In human mitochondria, mitochondrial Hsp70 (mortalin) and the nucleotide exchange factor (GrpEL1) work synergistically to stabilize proteins, assemble protein complexes, and facilitate protein import. In bacteria, mitochondria, and chloroplasts, the GrpE-family of NEFs interacts with substrate-bound Hsp70 to facilitate ADP and protein substrate release. Herein, we present structures of full-length human mortalin in a nucleotide-free and substrate-bound state in complex with full-length GrpEL1. To stabilize the complex for structural analysis, we introduced a point mutation, R126W, into mortalin (mortalinR126W) that is associated with EVEN-PLUS syndrome and has been shown to reduce mortalin’s ATPase activity and conformational flexibility.

Further refinement yielded a 2.96 Å resolution cryoEM map describing a complex consisting of full-length mortalinR126W bound to a protein substrate and a full-length GrpEL1 homodimer. Firstly, we observe an expanded NBD devoid of nucleotide that is mediated by extensive contacts with one protomer of GrpEL1, termed GrpEL1-A. Secondly, we detail the significant bending of the GrpEL1 α-helical stalk domain that enables interactions between the GrpEL1 stalk and mortalinR126W NBD and SBD. Finally, this structure provides insights into the interactions between the SBDα helical lid of mortalin and the second GrpEL1 protomer, GrpEL1-B. Critically, the lack of EM density within the nucleotide-binding pocket but strong density within the substrate-binding pocket suggests that our structure represents a previously unobserved intermediate state and suggests a step-wise mechanism for the nucleotide and substrate release action of GrpEL1. At the first interface, subdomain IB of the NBD contacts the β-wing domain of GrpEL1-A via a salt bridge between R107 in mortalinR126W and the carbonyl group of P172 in GrpEL1-A. Here, the mortalinR126W IDL is proximal to the GrpEL1 α-helical dimer with residues V435 and L438 within the hydrophobic IDL interacting with L82 in GrpEL1-B. Compared to the predicted GrpEL1 structure, our mortalinR126W-GrpEL1 structure exhibits a ~ 13° bending of the GrpEL1 α-helical domain. We observed strong density for a peptide bound to the SBD substrate binding pocket, indicating that our purified complex is substrate-bound. With these factors in mind, combined with Hsp70’s propensity to bind hydrophobic peptides, we modeled the bound peptide as VLLLDVT, corresponding to residues 435–441 of mortalin’s IDL region, into our cryoEM density. Second, we observe an interaction interface between the SBDα helical domain and the β-wing domain of GrpEL1-B. Here, Y173 from GrpEL1-B inserts itself into the mortalinR126W SBDα, forming electrostatic and cation-pi stacking interactions with R578 and R574, respectively.

> MASEAIKGAVVGIDLGTTNSCVAVMEGKQAKVLENAEGARTTPSVVAFTADGERLVGMPAKRQAVTNPNNTFYATKRLIGWRYDDPEVQKDIKNVPFKIVRASNGDAWVEAHGKLYSPSQIGAFVLMKMKETAENYLGHTAKNAVITVPAYFNDSQRQATKDAGQISGLNVLRVINEPTAAALAYGLDKSEDKVIAVYDLGGGTFDISILEIQKGVFEVKSTNGDTFLGGEDFDQALLRHIVKEFKRETGVDLTKDNMALQRVREAAEKAKCELSSSVQTDINLPYLTMDSSGPKHLNMKLTRAQFEGIVTDLIRRTIAPCQKAMQDAEVSKSDIGEVILVGGMTRMPKVQQTVQDLFGRAPSKAVNPDEAVAIGAAIQGGVLAGDVTDVLLLDVTPLSLGIETLGGVFTKLINRNTTIPTKKSQVFSTAADGQTQVEIKVCQGEREMAGDNKLLGQFTLIGIPPAPRGVPQIEVTFDIDANGIVHVSAKDKGTGREQQIVIQSSGGLSKDDIENMVKNAEKYAEEDRRKKERVEAVNMAEGIIHDTETKMEEFKDQLPADECNKLKEEISKMRELLARKDSETGENIRQAASS;>[2x]TLLEEKVKLEEQLKETVEKYKRALADTENLRQRSQKLVEEAKLYGIQAFCKDLLEVADVLEKATQCVPKEEIKDDNPHLKNLYEGLVMTEVQIQKVFTKHGLLKLNPVGAKFDPYEHEALFHTPVEGKEPGTVALVSKVGYKLHGRTLRPALVGVVKEASA;> VLLLDVT> MEVLDLVTGPDSVTEIEAFLNPRMGQPPTPESLTEGGQYYGWSRGINLATSDT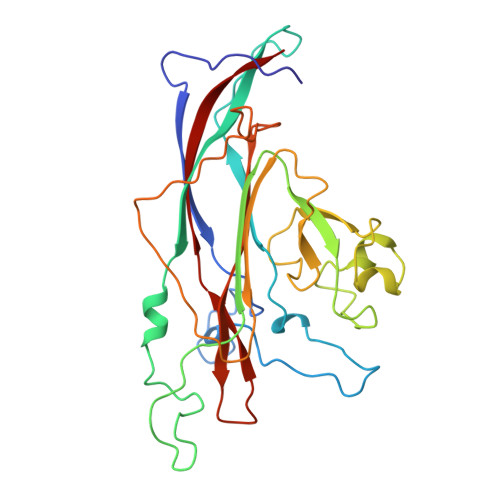EDSPGNNTLPTWSMAKLQLPMLNEDLTCDTLQMWEAVSVKTEVVGSGSLLDVHGFNKPTDTVNTKGISTPVEGSQYHVFAVGGEPLDLQGLVTDARTKYKEEGVVTIKTITKKDMVNKDQVLNPISKAKLDKDGMYPVEIWHPDPAKNENTRYFGNYTGGTTTPPVLQFTNTLTTVLLDENGVGPLCKGEGLYLSCVDIMGWRVTRNYDVHHWRGLPRYFKITLRKRWVK5'-O-[(S)-[(2-aminobenzoyl)oxy](hydroxy)phosphoryl]adenosine 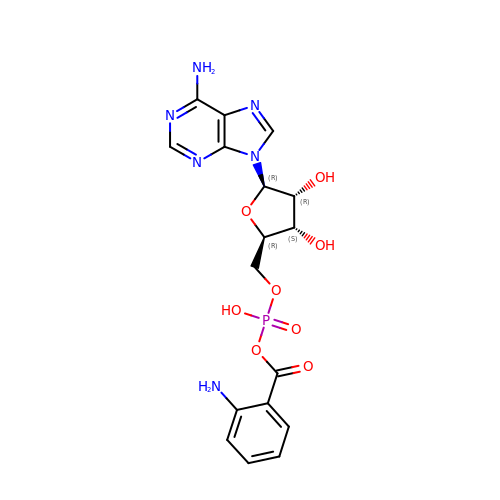| C17 H19 N6 O8 P | XZXXWUQOHYJTTC-XNIJJKJLSA-N> SHMPIQVLPPQLANQIAAGEVVERPASVVKELVENSLDAGATRIDIDIERGGAKLIRIRDNGCGIKKDELALALARHATSKIASLDDLEAIISLGFRGEALPSISSVSRLTLTSRTAEQQEAWQAYAEGRDMNVTVKPAAHPVGTTLEVLDLFYNTPARRKFLRTEKTEFNHIDEIIRRIALARFDVTINLSHNGKIVRQYRAVPEGGQKERRLGAICGTAFLEQALAIEWQHGDLTLRGWVADPNHTTPALAEIQYCYVNGRMMRDRLINHAIRQACEDKLGADQQPAFVLYLEIDPHQVDVNVHPAKHEVRFHQSRLVHDFIYQGVLSVL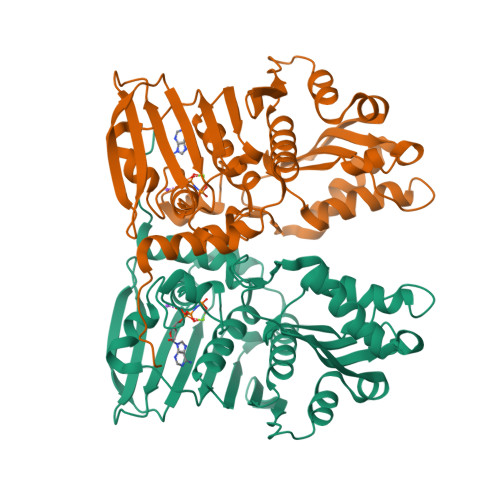Q>[2x]MEASVSFENGKIVVRLPITRPTSKIRVKKIENGVGIPVSTRKKSFPSDENLRDYYIEWQISFARDGKYDYELSRMVRLAHEHGILTYNDIYELL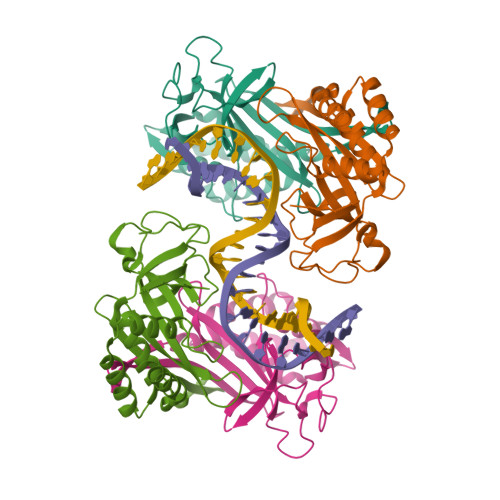KFADDVKSYLEDKGIRRESTNEELYGFNIYEDVYPVAKKELPSGEFIGIVLKHAQRAVGYQSMVYVCIPLTNVEPSLAGRVARRNEVVKYEVPVDLMKELLKAFIIASETHKNDIVKFLRSIIGTS>MTTTSPLHFVTLLGSLRKASFNAAVARALPEIAPEGIAITPLGSIGTFPHYSQDVQEEGFPAPVLTMAQQIATADAVVIVTPEYNYSVPGVLKNAIDWLSRVSPQPLAGKPVALVTASPGMIGGARAQYHLRQSLVFLDAYVLNRPEAMIGQVTGKVDAQTLELSDVATREFLARQLDALAALARTLSPRAITHHHHHH[4x]

Gh-ChrR belongs to the superfamily of NAD(P)H-dependent FMN reductases that catalyze the metabolic detoxification of quinones and their derivatives to hydroquinones, using NAD(P)H as the electron donor. This family of enzymes protects cells against quinone-induced oxidative stress, cytotoxicity, and mutagenicity in both prokaryotic and eukaryotic organisms. As expected from the sequence homology between Gh-ChrR and other members of the FMN reductase family (Pfam ID: PF03358), Gh-ChrR functions as a NAD(P)H–dependent metal reductase.

The crystal structure of Gh-ChrR was elucidated to a resolution of 2.25 Å. The crystallographic asymmetric unit contains four monomers, each with a single bound FMN. The homotetramer is assembled as two sets of identical dimers (cyan/yellow and blue/purple) that are aligned side-by-side with an approximately 60 degree angle along the parallel plane α4 and α5 of each dimer. The β-strands are organized into one parallel β-sheet, β2:β1:β3:β4:β5, flanked by helices α1 and α5 on one face and the remaining helices on the opposite face. FMN binds in a pocket on the surface of Gh-ChrR near the dimer interface. The negatively charged ribityl phosphate group of FMN is deeply buried in a positively charged region (blue) composed of residues in the loop between β1 and α1 (S15–N22) and a positive electrostatic dipole from the N-terminus of the capped α-helix (α1) similar to that previously reported. As a consequence, the active site of Gh-ChrR is open and solvent accessible, a feature observed at the active site of oxidoreductases that facilitates promiscuous exchange of substrates. While bound FMN is observed in the crystal structure of Gh-ChrR, NADH, an essential electron transfer component of the reductive reactions catalyzed by NAD(P)H-dependent FMN reductases, is absent. Regardless of the forces holding a negatively charged Cl− ion in place in Gh-ChrR, the side chain of R101 is a good candidate to assist the binding of an anion. Negatively charged species analogous to Cl−, including chromate, ferricyanide and uranyl ions, may be recruited to the catalytic center about R101 at a favorable distance (∼3.5 Å) for hydride transfer from FMNH2 to the metal.>MAKIIGGFAVSHTPTIAFAHDANKYDDPVWAPIFQGFEPVKQWLAEQKPDVTFYVYNDHMTSFFEHYSHFALGVGEEYSPADEGGGQRDLPPIKGDPELAKHIAECLVADEFDLAYWQGMGLDFGAFSPLSVLLPHEHGWPCRIVPLQCGVLQHPIPKARRFWNFGRSLRRAIQSYPRDIKVAIAGTGGLSHQVHGERAGFNNTEWDMEFMERLANDPESLLGATVTDLAKKGGWEGAEVVMWLLMRGALSPEVKTLHQSYFLPSMTAIATMLFEDQGDAAPPAESDEALRARAKRELAGVEEIEGTYPFTIDRAVKGFRINHFLHRLIEPDFRKRFVEDPEGLFAESDLTEEEKSLIRNRDWIGMIHYGVIFFMLEKMAAVLGIGNIDVYAAFRGLSVPEFQKTRNAAITYSVAGKQ[2x]

The three catecholic compounds are degraded by three evolutionarily related type II extradiol dioxygenases–DesB, LigAB, and DesZ–in S. sp. SYK-6. On the other hand, DesB exhibits not only a strict substrate specificity but also high enzyme activity for gallate. While LigAB is an α2β2-type tetramer, DesB is a β2-type homo-dimer. In this study, we analyzed the mechanism of the substrate recognition of DesB on the basis of the crystal structures of reaction intermediates.

His124, which is also conserved in type II dioxygenases, forms a hydrogen bond with OH of the substrate, which is an equatorial ligand of the Fe (II) ion. Earlier studies of extradiol dioxygenases suggested that His124 contributes to the deprotonation of the substrate by forming a hydrogen bond with OH. Since the His124Phe mutant shows no detectable enzyme activity (less than 0.01 U/mg), His124 is also indispensable to the enzyme activity for DesB. Furthermore, crystallographic analysis of this mutant showed that the His124Phe mutation is unlikely to affect the Fe (II) binding at the active site (see below). Crystal structure analysis of the anaerobic DesB (His124Phe)-gallate complex showed that the Fe (II) ion was located at the R-site. Gallate is bound to the active site of the mutant, and the carboxyl group of gallate forms hydrogen bonds with Asn387’ and Tyr391’. His124 and His192 function as catalytic acid and base for the ring-opening reaction, respectively.> PQFSLWKRPVVTAYIEGQPVEVLLDTGADDSIVAGIELGNNYSPKIVGGIGGFINTLEYKNVEIEVLNKKVRATIMTGDTPINIFGRNIL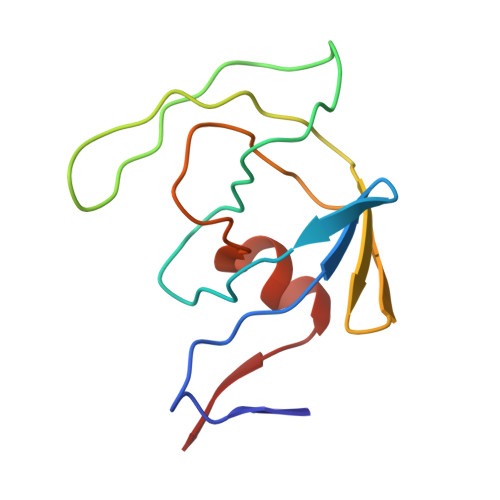TALGMSLNL1,3-dimethyl-1H-pyrrolo[3,4-d]pyrimidine-2,4(3H,6H)-dione 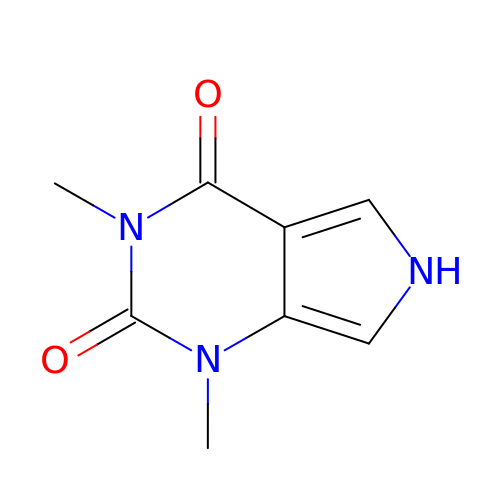| C8 H9 N3 O2 | MNPOFAXKBZPGNK-UHFFFAOYSA-N>[12x]SNADRLDVAMAADDICTAITNGEQVKGLYLYGPFGTGKSFILGAI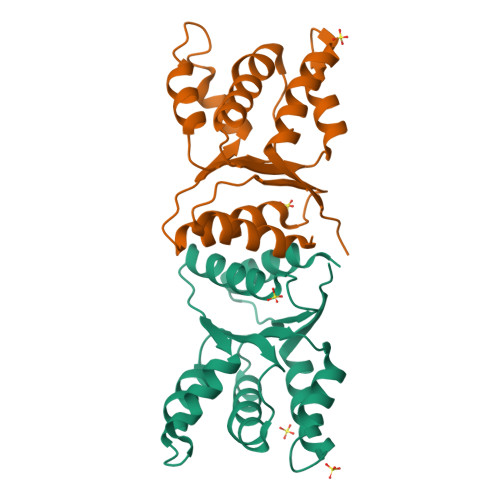ANQLKSKKVRSTIIYLPEFIRTLKGGFKDGSFEKKLHRVREANILMLDDIGAEEVTPWVRDEVIGPLLHYRMVHELPTFFSSNFDYSELEHHLAMTRDGEEKTKAARIIERVKSLSTPYFLSGENFRNN5-methoxy-N-[(5-methylpyridin-2-yl)sulfonyl]-1H-indole-2-carboxamide | C16 H15 N3 O4 S | 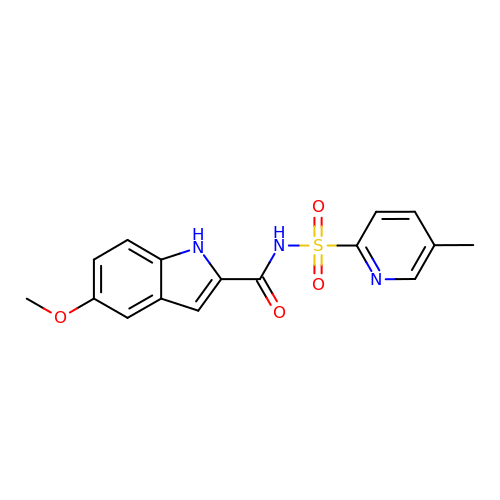ZKUFSBNJBIOKLO-UHFFFAOYSA-N>[2x]GSSGSSGMSVTYDDSVGVEVSSDSFWEVGNYKRTVKRIDDGHRLCSDLMNCLHERARIEKAYAQQLTEWARRWRQLVEKGPQYGTVEKAWMAFMSEAERVSELHLEVKASLMNDDFEKIKNWQKEAFHKQMMGGFKETKEAEDGFRKAQKPWAKKLKEVEAAKKAHHAACKEEKLAISREANSKADPSLNPEQLKKLQDKIEKCKQDVLKTKEKYEKSLKE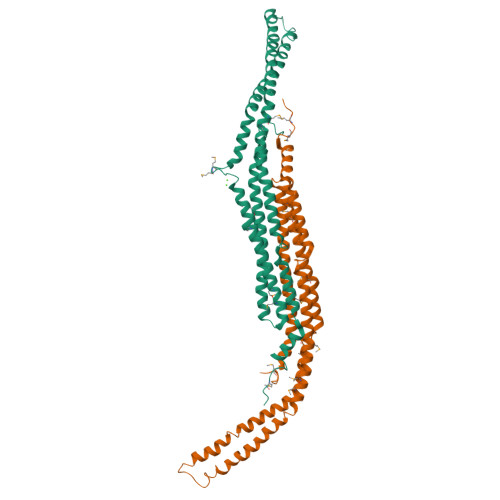LDQGTPQYMENMEQVFEQCQQFEEKRLRFFREVLLEVQKHLDLSNVAGYKAIYHDLEQSIRAADAVEDLRWFRANHGPGMAMNWPQFEEWSADLNRTLSRREKKKATDGVTLTGINQTGDQSLPSKPSS>XELAAIKEELAAIKXELAAIKQ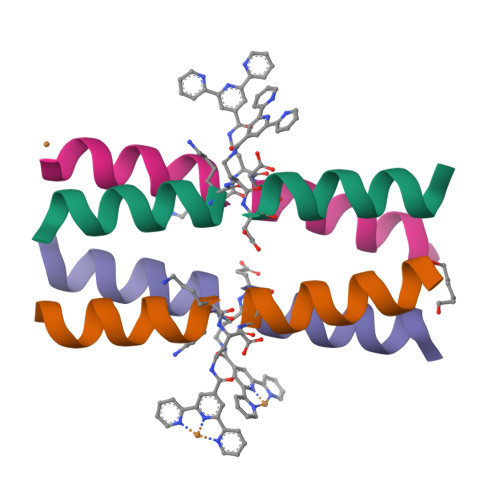ELAAIKQX[6x]4-{[5-hydroxy-6-(4-methylphenyl)pyrimidin-4-yl]amino}benzene-1-carboximidamide 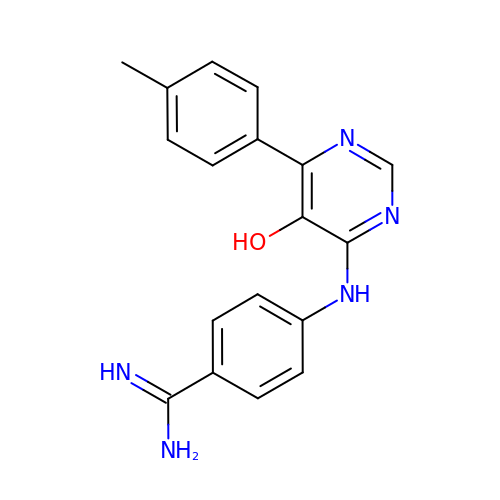| C18 H17 N5 O | FQSMNGLHSXWGEE-UHFFFAOYSA-N> MGKTYDVNICYA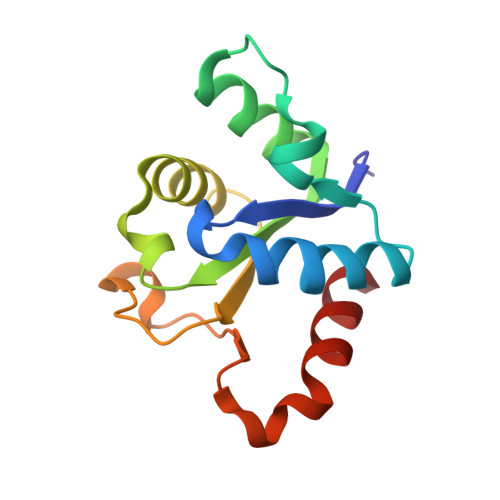PEDREWVINTLVFKLERAGIKTFVNIRDDTPGNFFAENIMDAIENSNRTIVVMSPDFFKNNICDKTLQIGLSHQIIPILYRPCEVPYFLNHMTYLDWCDKDVRPVFWRNLFRDIRNN>MEFDDDLVDAEGNLVEGGGTYYLLPHIWAHGGGIETAKTGNEPCPLTVVRSPNEVSKGEPIRISSQFLSLFIPRGSLVALGFANPPSCAASPWWTVVDSPQGPAVKLSQQKLPEKDILVFKFEKVSHSNIHVYKLLYCQHDEEDVKCDQYIGIHRDRNGNRRLVVTEENPLELV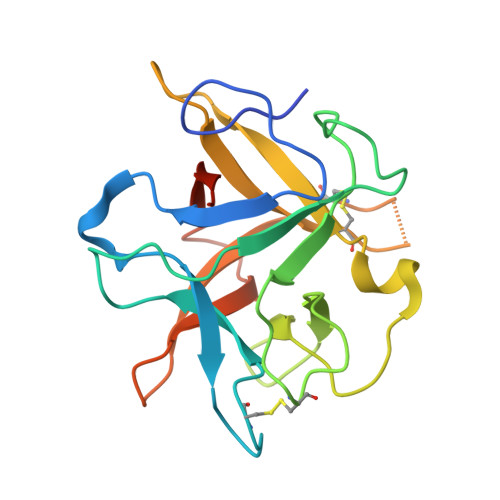LLKAKSETASSH[2x]2-(4-ethoxy-8-methylquinazolin-2-yl)guanidine | C12 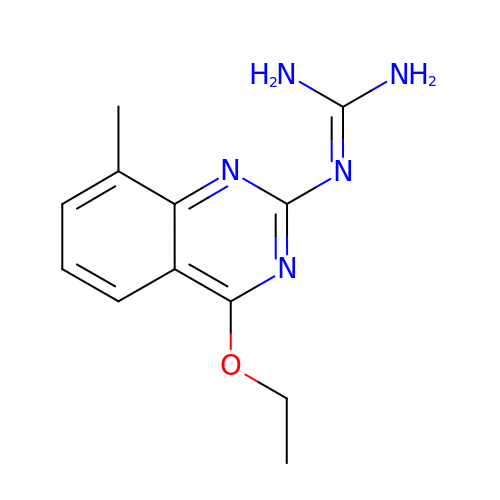H15 N5 O | FIIINVTXWYOJPG-UHFFFAOYSA-N>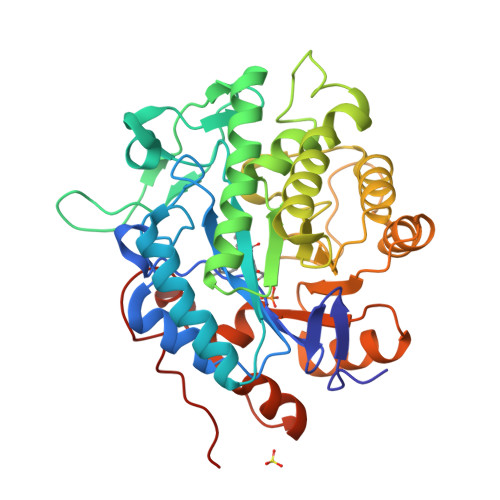[3x]MTSLFEPAQAGDIALANRIVMAPLTRNRSPGAIPNNLNATYYEQRATAGLIVTEGTPISQQGQGYADVPGLYKREAIEGWKKITDGVHSAGGKIVAQIWHVGRISHTSLQPHGGQPVAPSAITAKSKTYIINDDGTGAFAETSEPRALTIDDIGLILEDYRSGARAALEAGFDGVEIHAANGYLIEQFLKSSTNQRTDDYGGSIENRARFLLEVVDAVAEEIGAGRTGIRLSPVTPANDIFEADPQPLYNYVVEQLGKRNLAFIHVVEGATGGPRDFKQGDKPFDYASFKAAYRNAGGKGLWIANNGYDRQSAIEAVESGKVDAVAFGKAFIANPDLVRRLKNDAPLNAPNQPTFYGGGAEGYTDYPALAQHHHHHH>[3x]MLYEEDYKLALEAFKKVFNALTHYGAKQAFRSRARDLVEEIYNSGFIPTFFYIISKAELNSDSLDSLISLFSSDNAILRGSDENVSYSAYLFIILYYLIKRGIIEQKFLIQALRCEKTRLDLIDKLYNLAPIISAKIRTYLLAIKRLSEALIEAR;>MPYYAFAEPFFIHAITHLHVGSGSSVEEEIALPFQRDELGYPTIYASSLKGAIKSFLLKEFPDKRDVIYKVLGEDENPEEASLGTFLDAILFAIPSRIIEIDSAKPYVWVYVTTYELLKKVKLYLDSISQLSNASFSNLKNKIDTILAKEGKNITLDSDLKSAILNEDFYVELEALNNKIPSIINAGVPLLVLEDSIGREVINRSLIRVRRIRIDRDKKVVETGGLWSEEYVPMKTIFFSVLLGKESKESAIFASCILRNLRYVILGGKETIGKGIVELRWVKDVI[4x];> MKRVLIKPLEPLMFRSQGEFEPLITGSHTAAQSLIIPRPSTIAGMLGYILFNKSSGTGDWLSDLTNLLATIYGTFIETNGEYLFPLRMGNHLALVDQQHLINLPTLLEKEYERREKGIYELFYDKNKLFQIINHQDRIGISIDKSTRTVKEHYLYSARYLAFKKEVNYVIFIDNDAISDKINGKIVNFGGENRIAKLEVDDYKVDTSIEEEYYLALSPILIPDEALDNFLDNISDYVAMGKVDKISLGFDIANTKRKEMLTAILEGSIVKRSIIDFIKNEIKNDLRYRFSKYEKIGYNTLMSLCKLALRKILS;> MAIDFLVNILELIKEKQCNINLFSAISLTSIVYNNFGEFLSNNQSYSTNNPLLKYHIIILNDKNKTKDVEEKRNIFKREVAELISRNFKLDGEKVRNYFDSLKEVLKSLKYTIVDVEITTRTRALIGVSTSLGKLIFGSGISFDPYMNLPYIPASEIKGIVRSYIEGKLGEQEAEEIFGNEEREGNVNFTDAYPTRSKDFLFVPDVITPHYNGKKSEADAEPRPVIHLTIAPKVTFRFLIYYKREDVGKPICDSMPIILIRGLGARSSVGYSLFELRKIEVIKAAAHHHHHHHHHH;> MEELLMSLKLKALYPLTGGYNRHSINPFYEELVRPTEIKGLWRWWNRVLFNTLAYSTKGKLYTYE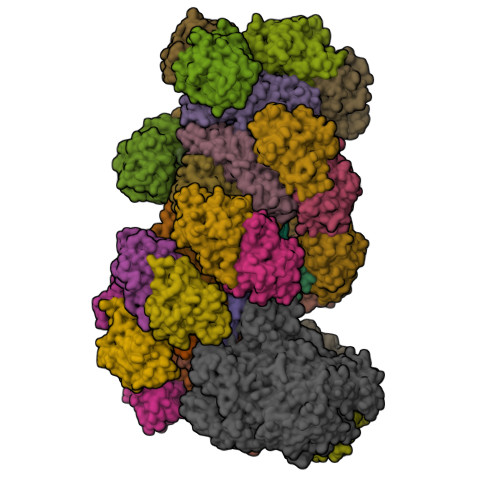SIDRLFEDVFGSENKKSAVRLEVITDEGNDNRFELSYVELDKVIDCLRNYKRKVSLDFIDNTLIAEIEGSTKIPISFKSNLDIDKIIKDLVHNNKLLSFELLGFKSVEIDATKISDKKILKEILRDLITNYLEYFNIKQEVTFTLNIYLDKSREHKQNFEDKLKFALYSLLVFILLGGIGRKTSRGFGSLSIIDVKCYDNSICKKIEDLAKNFLKISSGNELKSKIESILDCIKNSCIDTLYIENNILSEIDPKKNVVYFINSDLFEVKRINDKEKVLANIYKAVSSEGCCIKSIITDKYVRKSFLIAFGGYRKVEKDKGLDIGFIKNYLCETCETVSSFNIVDFLLSEGSFMSDYILQYEHRNSLLRFKLISDNSNNSYLIGYILHSSYFKKIDIKYVRCILEKLTYCVI;> MSIDNVLREFLDYKIIALLHDPPNKAWVITGRARNLTQQLSNIRASRKHEKVAKYIINQLFGKNYSEKVDNADKLASSIDRYLGSIVYKERSLFENRSIFLKNILLSNIQRDIGNLFPKDKSKLDNLILEYKKLLNVINKTNLILKYQLFYLIYELVWIDSKYENTPSDTRNPTHTIFDHLYATAAMMNWILSLEKEAKGYLLGIDTIGVADFISKGRKTRDLWISSYLVSALLWYVITWFIEEYGPDVILFPSLRFNQFYAFYLLEKLRKEGVSEDVIDEIKELITKYIFNGDDLFENLKIPPYPIIPGRITLILPGLIREGEEYKKVQDDNCFISKVKERYNEGWRKLIEGLRCYSERKREDGFWNLVCRVLKLTEDLLQTTPLNIRVKQVSVTEDEIFNNNKLRSDSWKIYDNKYRQLVSEFKKSKLVKVTPESRLKLFELTKFDKLPQIGEKSKRGYEFCTSCGVLPAVVIMPKEDELEKKLIDLGIARDEKDVRSIKNMISPGERLCPWCLVKRALGAEPRLMRILLLGDLYSVEKIVNEIVSRDVKIEIPSTSDIASIKTFEEMIEKKNEICEDLKEEEVCEKPSESVLSMWQWFNKNYYNGINLTIDPEEYWFSEKRRRYYFSVFRRHRITFPSPYYALVRADSDYLGDLLEGKLTPYLAGIIDSGDYANISEKKEEVNKLLEEYLVNAGSGSIVDYVKTVLKCIRENLNKCSCAEKIYSNEVAKVMFRVNVEKANVEEEVKNSLEYFETILNEGRIIVTPAWHVSISSALNRGLLVELELVNKHKGFVIYAGGDDLLAMLPVDEVLDFIKESRRAFAGFGTEKLGNMCLENGFVRINNAYYPSLPIVGRSYSVIIAHYADPLFFVINDSYNLLEEGKEIIRYRVMYNGEYKDAKKDVAIFRYQGLTSVIPLSLKRPIVSSVSDFNEIASIIDVILELKKRIDEGRISVSLLYDYEKYKHLIVASDEKYLTEFLVKDWIKRNSLRKHVEFTIDEKLYGVRLTIENYPIKIPNDLISNIVYTLRIIYGGEK;>MSTQREYVFIPITNSITIDVKITIGGSDHITNIDERGIHNVLVITGYAVDEKNGRLVPTLDPCDYVKGILVAGTPQQAQSNDFLTLKLPANKLYLIRKKGNISDDLKIYIPYSSPDARNSMKTKPVSISDDTIVNNIIKEVFDKIYNITQKEKVKIEKVKEDIKELFSYYALEQ[22x]>[2x]MVNPTPPPSLEDAA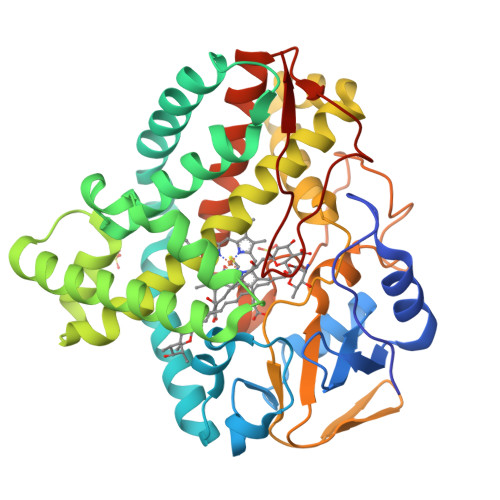PSVLRLSPLLRELQMRAPVTKIRTPAGDEGWLVTRHAELKQLLHDERLARAHADPANAPRYVKSPLMDLLIMDDVEAARAAHAELRTLLTPQFSARRVLNMMPMVEGIAEQILNGFAAQEQPADLRGNFSLPYSLTVLCALIGIPLQEQGQLLAVLGEMATLNDAESVARSQAKLFGLLTDLAGRKRAEPGDDVISRLCETVPEDERIGPIAASLLFAGLDSVATHVDLGVVLFTQYPDQLKEALADEKLMRSGVEEILRAAKAGGSGAALPRYATDDIEIADVTIRTGDLVLLDFTLVNFDEAVFDDADLFDIRRSPNEHLTFGHGMWHCIGAPLARMMLKTAYTQLFTRLPGLKLASSVEELQVTSGQLNGGLTELPVTW>[2x]SNAMETFLFTSESVNEGHPDKLCDQISDAVLDACLEQDPDSKVACETCTKTNMVMVFGEITTKATIDYEKIVRDTCRSIGFISDDVGLDADKCKVLVNIEQQSPDIAQGVHGHFTKRPEDIGAGDQGHMFGYATDETPELMPLSHVLATKIGARLTEVRKNGTCRWLRPDGKTQVTVEYYNDNGAMVPVRVHTVLISTQHDETVTNDEIARDLKEHVIK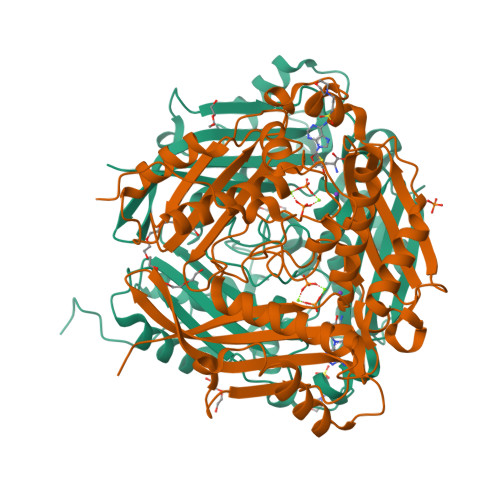PIIPEKYLDDKTIFHLNPSGRFVIGGPHGDAGLTGRKIIIDTYGGWGAHGGGAFSGKDPTKVDRSGAYIVRQAAKSVVANGMARRALVQVSYAIGVPEPLSVFVDTYGTGLIPDKEILKIVKETFDFRPGMMTINLDLKRGGNGRFQKTAAYGHFGRDDPDFTWEVVKPLKWDKPQLNNIGSG> MGNVDLVFLFDGSMSLQPDEFQKILDFMKDVMKKLSNTSYQFAAVQFSTSYKTEFDFSDYVKRKDPDALLKHVKHMLLLTNTFGAINYVATEVFREELGARPDATKVLIIITDGEATDSGNIDAAKDIIRYIIGIGKHFQTKESQETLHKFASK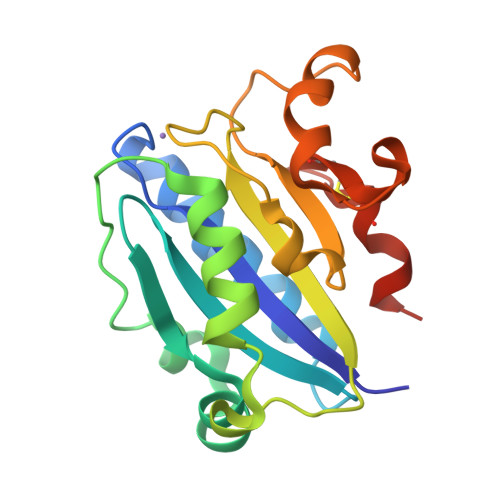PASEFVCILDTFECLKDLFTELQKKI>TFAGDNGTMMQYFEWYLPNDGTLWTKMGSDASHLKSIGITGVWFPPAYKGQSQSDVGYGVYDMYDLGEFNQKGTVRTKYGTKAQLQSAITSLHNNGIQAYGDVVLNHRMGADATETISAVEVNPSNRNQVTSGAYNISAWTDFEFPGRGNTYSSFKWHSYYFDGVDWDQSRQLSGKIYQIQGKAWDWEVDSENGNYDYLMGADIDYDHPDVQTEVKNWGKWFVNTLNLDGVRLDAVKHIKFDYMSSWLSSVKSTTGKSNLFAVGEYWNTSLGALENYENKTNWSMSLFDVPLHMNFQAAANGGGYYDMRNLLNNTMMKNHPIQAVTFVDNHDTEPGQALQSWVSDWFKPLAYATILTRQ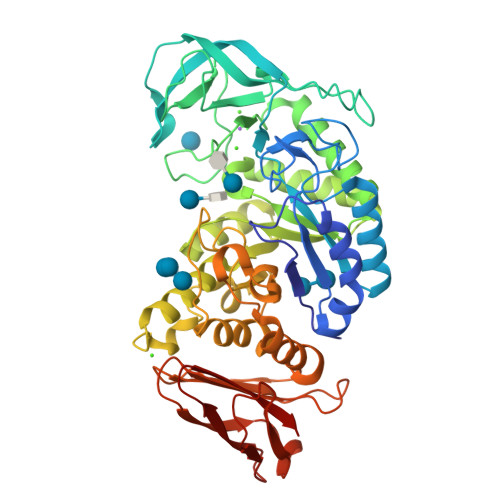EGYPCVFYGDYYGIPSQSVSAKSTWLDKQLSARKSYAYGTQHDYLDNQDVIGWTREGDSAHAGSGLATVMSDGPGGSKTMYVGTAHAGQVFKDITGNRTDTVTINSAGNGTFPCNGGSVSIWVKQ[2x]>ATVGPRVIVVGAGMSGISAAKRLSEAGITDLLILEATDHIGGRMHKTNFAGINVELGANWVEGVNGGKMNPIWPIVNSTLKLRNFRSDFDYLAQNVYKEDGGVYDEDYVQKRIELADSVEEMGEKLSATLHASGRDDMSILAMQRLNEHQPNGPATPVDMVVDYYKFDYEFAEPPRV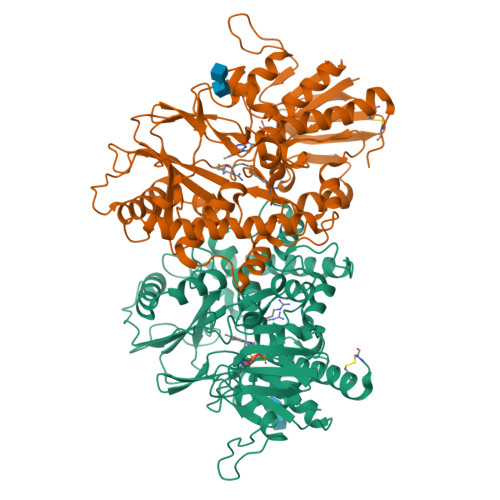TSLQNTVPLATFSDFGDDVYFVADQRGYEAVVYYLAGQYLKTDDKSGKIVDPRLQLNKVVREIKYSPGGVTVKTEDNSVYSADYVMVSASLGVLQSDLIQFKPKLPTWKVRAIYQFDMAVYTKIFLKFPRKFWPEGKGREFFLYASSRRGYYGVWQEFEKQYPDANVLLVTVTDEESRRIEQQSDEQTKAEIMQVLRKMFPGKDVPDATDILVPRWWSDRFYKGTFSNWPVGVNRYEYDQLRAPVGRVYFTGEHTSEHYNGYVHGAYLSGIDSAEILINCAQKKMCKYHVQGKYD[3x]>[4x]MYKDLEGKVVVITGSSTGLGKSMAIRFATEKAKVVVNYRSKEDEANSVLEEIKKVGGEAIAVKGDVTVESDVINLVQSAIK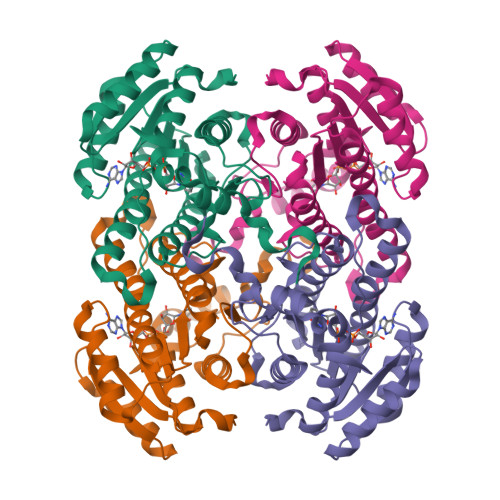EFGKLDVMINNAGLENPVSSHEMSLSDWNKVIDTNLTGAFLGSREAIKYFVENDIKGTVINMSSVHEKIPWPLFVHYAASKGGMKLMTETLALEYAPKGIRVNNIGPGAINTPINAEKFADPEQRADVESMIPMGYIGEPEEIAAVAAWLASSEASYVTGITLFADGGMTLYPSFQAGRG> GPGYQDPKGRLYGTIGIQKRFYVSIDKIPEHVINAFVATEDRNFWHHFGIDPVAIVRAAIVNYRAGRIVQGGSTITQQLAKNLFLTRERTLERKIKEALLAIKIERTFDKKKIMELYLNQIYLGSG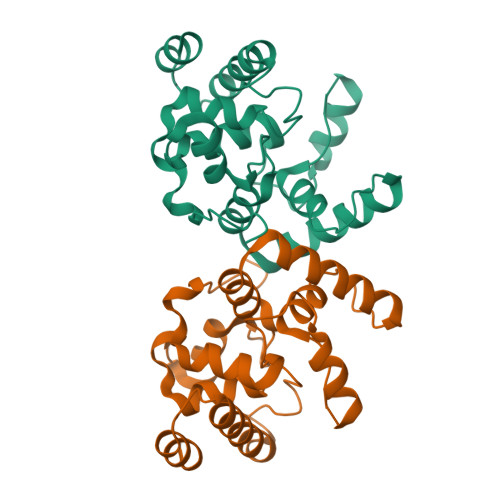AYGVEAAAQVYFGKHVWELSLDEAALLAALPKAPAKYNPFYHPERALQRRNLVLKRMLEEGYITPEQYEEAVNK> EKVDNPFEGAKLYVNPVWSAKAAAEPGGSAVANESTAVWLDRIGAIEGNDSPTTGSMGLRDHLEEAVRQSGGDPLTIQVVIYNLPGRDCAALASNGELGPDELDRYKSEYIDPIADIMWDFADYENLRIVAIIEIASLPNLVTNVGGNGGTELCAYMKQNGGYVNGVGYALRKLGEIPNVYNYIDAAHHGWIGWDSNFGPSVDIFYEAANASGSTVDYVHGFISNTANYSATV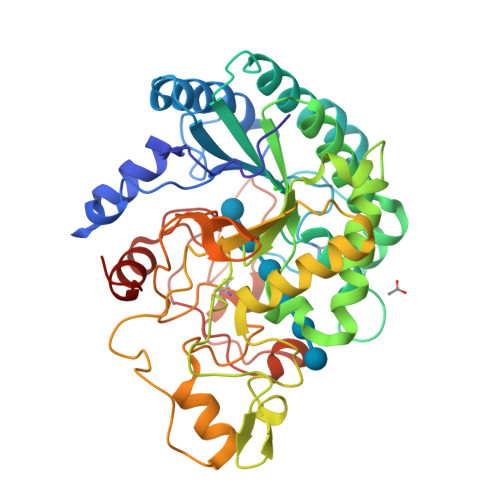EPYLDVNGTVNGQLIRQSKWVDWNQYVDELSFVQDLRQALIAKGFRSDIGMLIDTSRNGWGGPNRPTGPSSSTDLNTYVDESRIDRRIHPGNWCNQAGAGLGERPTVNPAPGVDAYVWVKPPGESDGASEEIPNDEGKGFDRMCDPTYQGNARNGNNPSGALPNAPISGHWFSAQFRELLANAYPPL> ADQRRDFIDIESKFALRTPEDTAEDTCHLIPGVAESVATCHFNHSSKTFMVIHGWTVTGMYESWVPKLVAALYKREPDSNVIVVDWLSRAQEHYPVSAGYTKLVGQDVARFINWMEEEFNYPLDNVHLLGYSLGAHAAGIAGSLTNKKVNRITGLDPAGPNFEYAEAPSRLSPDDADFVDVLHTFTRGSPGRSIGIQKPVGHVDIYPNGGTFQPGCNIGEAIRVIAERGLGDVDQLVKCS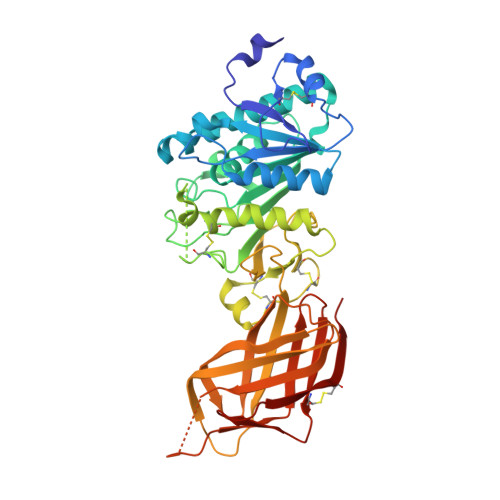HERSIHLFIDSLLNEENPSKAYRCSSKEAFEKGLCLSCRKNRCNNLGYEINKVRAKRSSKMYLKTRSQMPYKVFHYQVKIHFSGTESETHTNQAFEISLYGTVAESENIPFTLPEVSTNKTYSFLIYTEVDIGELLMLKLKWKSDSYFSWSDWWSSPGFAIQKIRVKAGETQKKVIFCSREKVSHLQKGKAPAVFVKCHDKSLNKKSG>MDDNPTAVKLDQGGNQAPQGRGRRCLPKALGYITGDMKEFANWLKDKPQALQFVDWVLRGISQVVFVSNPISGILILVGLLVQNPWCALNGCVGTVVSTLTALLLSQDRSAITAGLQGYNATLVGILMAIYSDKGNYFWWLLFPVSAMSMTCPVFSSALNSVLSKWDLPVFTLPFNMALSMYLSATGHYNPFFPSTLITPVTSVPNVTWPDLSALQLLKSLPVGVGQIYGCDNPWTGGIFLGAILLSSPLMCL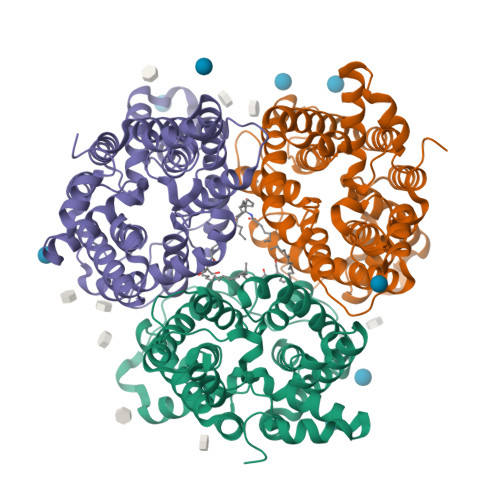HAAIGSLLGIIAGLSLSAPFEDIYAGLWGFNSSLACIAIGGTFMALTWQTHLLALACALFTAYLGASMSHVMAVVGLPSGTWPFCLATLLFLLLTTKNPNIYKMPISKVTYPEENRIFYLQSRKRTVQGPL[3x]>[2x]GSFKFTAQQHVYDINGVKVGGQPGEYPTVLIGSIFYRGHKIVSDGQKGIFDKDAAKALLDQEAELSAETGNPFIIDVLGESVEALTKYVEFILENTTAPFLLDSISPDVRVGALKNLGKDPEIQKRLIYNSIEEHYTEEELAA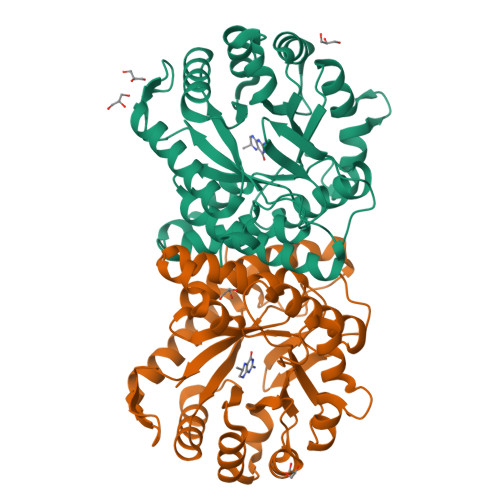IKEAGLKTAVILAFSKKALKPNARIDLLQGKDDKEGLIAAAKRAGIEQFLVDPGVLDVASNSWTTEAINVVKEQFGYPGGCAPSAAVYLWKKMRSKGTPFFEVAGAAVFTYPITQGADFILYGPMMNAPWVYRAIATTDAMIAYNNKLTGVKMGTTEHPLLKIF> GSMPKPINVRVTTMDAELEFAIQPNTTGKQLFDQVVKTVGLREVWFFGLQYVDSKGYSTWLKLNKKVTQQDVKKENPLQFKFRAKFFPEDVSEELIQEITQRLFFLQVKEAILNDEI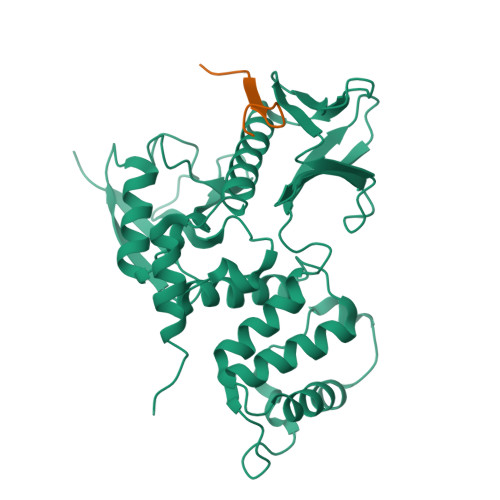YCPPETAVLLASYAVQAKYGDYNKEIHKPGYLANDRLLPQRVLEQHKLTKEQWEERIQNWHEEHRGMLREDSMMEYLKIAQDLEMYGVNYFEIKNKKGTELWLGVDALGLNIYEHDDKLTPKIGFPWSEIRNISFNDKKFVIKPIDKKAPDFVFYAPRLRINKRILALCMGNHELYMRRRKPDTIEVQQMKAQARVDSSGRIVTD;> RQRQKRRTGALTLSGGGKRN> GPL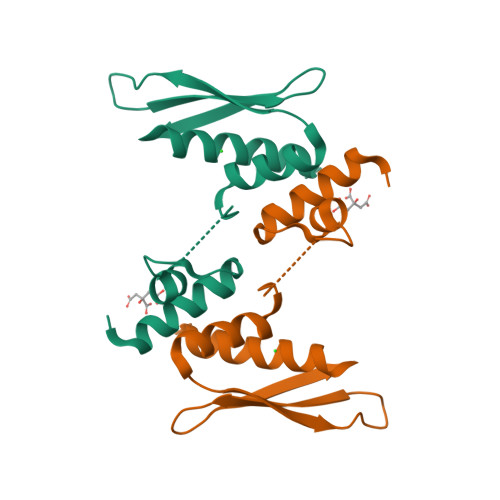GSKATVTAMIARELLYGGTSPTAETILKNNISSGHVPHGPLTRPSEQLDYLSRVQGFQVEYKDFPKNNKNEFVSLINCSSQPPLISHGIGKDVESCHDMAALNILKLLSELD> MAALVKPAGDTNVKTYPVMVDSRAYDKNGNYLGHMYYAYDNIDIVPTVVTINGKTYYKVANKDEYVRVTNITGNQRTLKHNAYIYWSSYRRTPGTGKMYRGQTVTTYGPQMKFKNGKKYYRIEGCRNNNKRYIKAVNFYHHHHHH

S-layer proteins (SLPs) are self-assembling, crystalline proteins coating the cell surfaces of many prokaryotes. We determined the atomic resolution structures of all functional domains (I-III from N- to C-termini) present in the three S-layer proteins SlpA_ac, SlpX_ac, and SlpA_amy. The Lactobacillus S-layers are anchored to the cell wall through interaction with teichoic acids (TA), either lipoteichoic acid (LTA) or wall teichoic acid (WTA).

The full-length SlpX_ac shows differences in structure and domain arrangement compared to the SlpA architecture. SlpX_ac_III is structurally highly conserved compared to SlpA_ac_III and SlpA_amy_III, whereas the sequence is less conserved (37 to 41% identity, 52 to 56% similarity). The crystal structures of the TAB domains (SlpA_ac_III, SlpA_amy_III, and SlpX_ac_III) reveal high structural similarities. The general structure of the TAB domain consists of two cell wall binding motifs (SlpA_motif) which are connected by a short linker and arranged as an internal homodimer. Mapping of the surface charges indicates a large, highly positively charged region within the interface of the two motifs that extends to the C-terminal part of the protein. The TAB domain (SlpX_ac_III) would still face inward and anchor the S-layer to the cell wall analogously to the SlpA-only layer.>HMVSEVRKKKLLHVFTVFFDSDKSGVVEKQDFELAAQNIAKLRGWAPGSPAYDILQESMIAIWLGLQKQADADGDGKVTQDEWLALWDEYAKDPAAAKDWQNLLCKSIFQIQDSSNDGSVDVNEYVTVHESFGLNKEESTEAFKKLAKGKDSISWADFQELWKEYFSSDDPDVPGNYIFGRLTC[6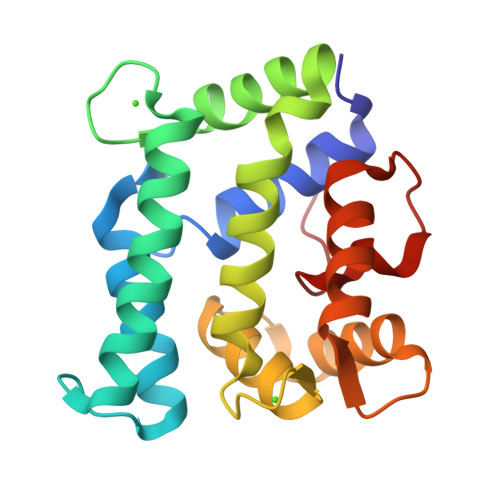x]> GHMSGSNTEEEIRMELSPDLISACLALEKYLDNPNALTERELKVAYTTVLQEWLRLACRSDAHPELVRRHLVTFRAMSARLLDYVVNIADSNGNTALHYSVSHANFPVVQQLLDSGVCKVDKQNRAGYSPIMLTALATLKTQDDIETVLQ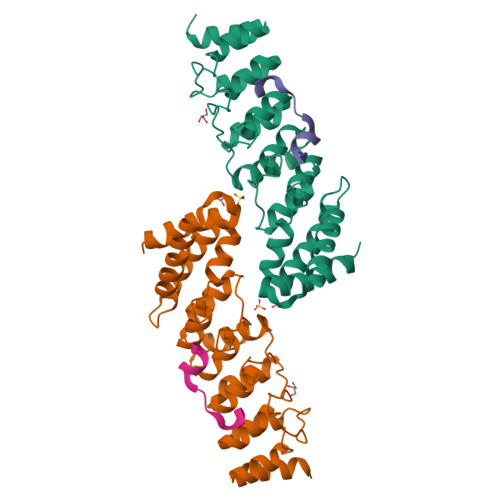LFRLGNINAKASQAGQTALMLAVSHGRVDVVKALLACEADVNVQDDDGSTALMCACEHGHKEIAGLLLAVPSCDISLTDRDGSTALMVALDAGQSEIASMLYSRMNIK;> GHMGHMSGSNTEEEIRMELSPDLISACLALEKYLDNPNALTERELKVAYTTVLQEWLRLACRSDAHPELVRRHLVTFRAMSARLLDYVVNIADSNGNTALHYSVSHANFPVVQQLLDSGVCKVDKQNRAGYSPIMLTALATLKTQDDIETVLQLFRLGNINAKASQAGQTALMLAVSHGRVDVVKALLACEADVNVQDDDGSTALMCACEHGHKEIAGLLLAVPSCDISLTDRDGSTALMVALDAGQSEIASMLYSRMNIK;>EVKPKNKARRRTTTQMELLYAD[2x]>[2x]GAMAKGAVTKLKFNSPIISTSDQLISTNELLDRLKALHEELASLDQDNTDLTGLDKYRDALVSRKLLKHKDVGIRAFTACCLSDILRLYAPDAPYTDAQLTDIFKLVLSQFEQLGDQENGYHIQQTYLITKLLEYRSIVLLADLPSSNNLLIELFHIFYDPNKSFPARLFNVIGGILGEVISEFDSVPLEVLRLIFNKFLTYNPNEIPEGLNVTSDCGYEVSLILCDTYSNRMSRHLTKYYSEIIHEATNDDNNSRLLTVVVKLHKLVLRLWETVPELINAVIGFIYHELSSEN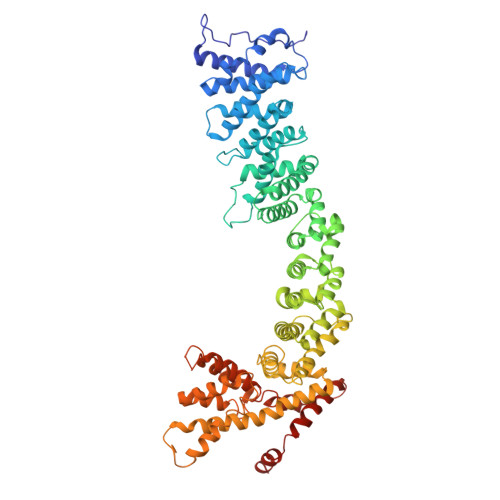ELFRKEATKLIGQILTSYSDLNFVSTHSDTFKAWISKIADISPDVRVEWTESIPQIIATREDISKELNQALAKTFIDSDPRVRRTSVMIFNKVPVTEIWKNITNKAIYTSLLHLAREKHKEVRELCINTMAKFYSNSLNEIERTYQNKEIWEIIDTIPSTLYNLYYINDLNINEQVDSVIFEYLLPFEPDNDKRVHRLLTVLSHFDKKAFTSFFAFNARQIKISFAISKYIDFSKFLNNQESMSSSQGPIVMNKYNQTLQWLASGLSDSTKAIDALETIKQFNDERIFYLLNACVTNDIPFLTFKNCYNELVSKLQTPGLFKKYNISTGASIMPRDIAKVIQILLFRASPIIYNVSNISVLLNLSNNSDAKQLDLKRRILDDISKVNPTLFKDQIRTLKTIIKDLDDPD>[2x]MASSAQDGNNPLFSPYKMGKFNLSHRVVLAPMTRCRALNNIPQAALGEYYEQRATAGGFLITEGTMISPTSAGFPHVPGIFTKEQVREWKKIVDVVHAKGAVIFCQLWHVGRASHEVYQPAGAAPISSTEKPISNRWRILMPDGTHGIYPKPRAIGTYEISQVVEDYRRSALNAIEAGFDGIEIHGAHGYLIDQFLKDGINDRTDEYGGSLANRCKFITQVVQAVVSAIGADRVG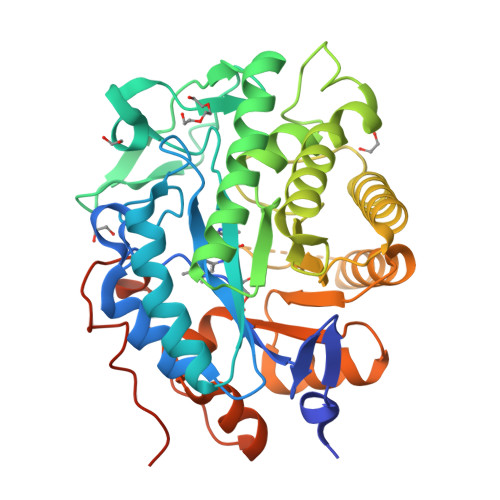VRVSPAIDHLDAMDSNPLSLGLAVVERLNKIQLHSGSKLAYLHVTQPRYVAYGQTEAGRLGSEEEEARLMRTLRNAYQGTFICSGGYTRELGIEAVAQGDADLVSYGRLFISNPDLVMRIKLNAPLNKYNRKTFFTQDPVVGYTDYPFLQGNGSNGPLSRLLEHHHHHH> HHHHHHMIVLFVDFDYFYAQVE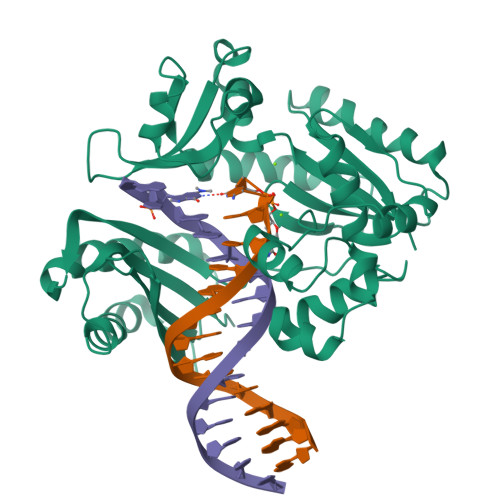EVLNPSLKGKPVVVCVFSGRFEDSGAVATANYEARKFGVKAGIPIVEAKKILPNAVYLPMRKEVYQQVSSRIMNLLREYSEKIEIASIDEAYLDISDKVRDYREAYNLGLEIKNKILEKEKITVTVGISKNKVFAKIAADMAKPNGIKVIDDEEVKRLIRELDIADVPGIGNITAEKLKKLGINKLVDTLSIEFDKLKGMIGEAKARYLISLARDEYNEPIRTRVRKSIGRIVTMKRNSRNLEEIKPYLFRAIEESYYKLDKRIPKAIHVVAVTEDLDIVSRGRTFPHGISKETAYSESVKLLQKILEEDERKIRRIGVRFSKFIEAIGLDKFFDT;> HHHHHHMIVLFVDFDYFYAQVEEVLNPSLKGKPVVVCVFSGRFEDSGAVATANYEARKFGVKAGIPIVEAKKILPNAVYLPMRKEVYQQVSSRIMNLLREYSEKIEIASIDEAYLDISDKVRDYREAYNLGLEIKNKILEKEKITVTVGISKNKVFAKIAADMAKPNGIKVIDDEEVKRLIRELDIADVPGIGNITAEKLKKLGINKLVDTLSIEFDKLKGMIGEAKAKYLISLARDEYNEPIRTRVRKSIGRIVTMKRNSRNLEEIKPYLFRAIEESYYKLDKRIPKAIHVVAVTEDLDIVSRGRTFPHGISKETAYSESVKLLQKILEEDERKIRRIGVRFSKFIEAIGLDKFFDT2-{HYDROXY[2-NITRO-4-(TRIFLUOROMETHYL)PHENYL]METHYLENE}CYCLOHEXANE-1,3-DIONE 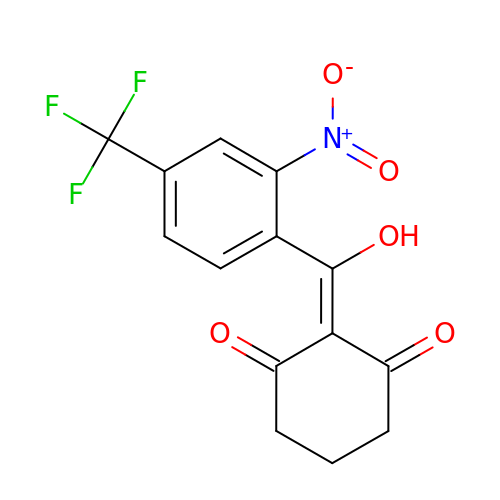| C14 H10 F3 N O5 | PMHVFNYNPNKNRO-UHFFFAOYSA-N>MKHHHHHHPMSDKIIHLTDDSFDTDVLKADGAILVDFWAEWCGPCKMIAPILDEIADEYQGKLTVAKLNIDQNPGTAPKYGIRGIPTLLLFKNGEVAATKVGALSKGQLKEFLDANLAGSAMESTVMVLRNMVDPKDIDDDLEGEVTEECGKFGAVNRVIIYQEKQGEEEDAEIIVKIFVEFSIASETHKAIQ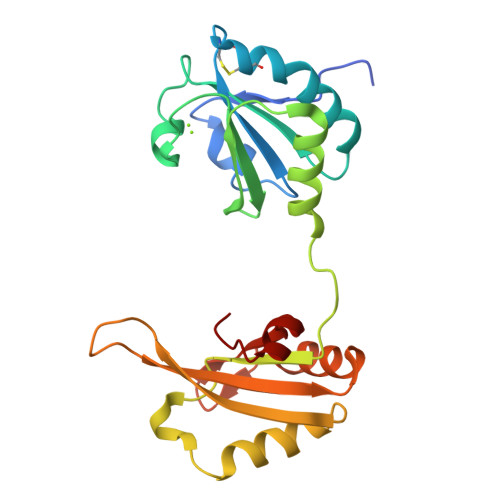ALNGRWFAGRKVVAEVYDQERFDNSDLSA[4x]> GPHMGAYWMSPTADDIRAMNRMQRQRVVGFTVGRENVGSVQFKVPVDLSNINLDDLFGTIVILEPRSATVYPNAAKKPPMGKGLNVPALISLEHSWPRGGPTIKGRRLERHIERLKSIPDTTFESYDPETGVWAFSVEHF;> MPKIKSFAPAWLNEPAPGHKLFAPAADDGTATVPLAYGKKIKPGPRRTIARRGTEIFVACGKQIRWGDLAQLKESWESRPSRSSVGPTSTKKDSSDFDDGAATAGYRIIKTPVADDIRQLVMSPNQDFLAVLTSHTVHICILPDSSHLHIQDTTPFKPKFWTLGPTTHVTSRSAVVSAVWHPLGVNGHALV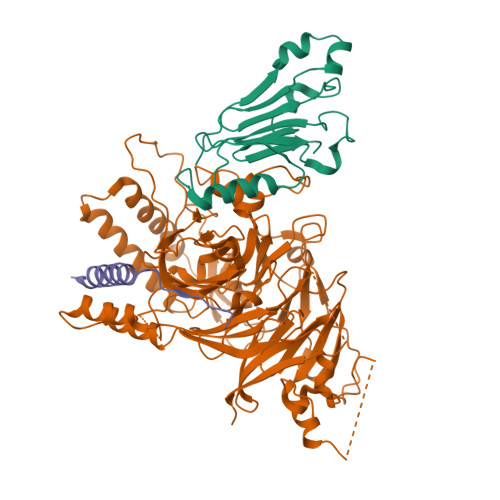TVTEDAIVRVWELSTADRWTFDAPTLAIDLKKLADATYLDQDFGVSTSATNKGFSPDAFDMEVAAACFPTRDSGGWAPMTLWLAMTSGDVYALCPLLPQRWTPPPTLIPSLSASIVAKVAAAEDNPESTPEERLVAQQQLEWMSEIDNQEPKLVEEATGEATIEVYTRPSRPGLVPKLQGPFDFDLNPEDEQDDEVELKDIYVIGEKPRVADLMRGEEEELEMMKEDQHNGLSLNIICLLSTSGQVKICLDIDGVEAQWLPPRSKNKRLFAPPPEPPSLLTFQTFDTLKPAEVTPDGWPMFSEDATSPYSFYVTHPAGITYISLTPWVFRLESELQSDSEAGTEFRIDLLAKGQGSERDRIFTQTRTQSPLAAATSIDDPDLGYFILSATQTDPIALFFETPER;> LRAREAKRKATLRMLRESLARVGPNVVRLRDD>SGSVTAGMALAATDIPGLDASKLVSGVLAEQRLPVFARGLATAVSNSSDPNTATVPLMLTNHANGPVAGRYFYIQSMFYPDQNGNASQIATSYNATSEMYVRVSYAANPSIREWLPWQRCDIGGSFTKEADGELPGGVNLDSMVTSGWWSQSFTAQAASGANYPIVRAGLLHVYAASSNFIYQTYQAYDGESFYFRCRHSNTWFPWRRMWHGGDFNPSDYLLKSGFYWNALPGKPATFPPSAHNHDVGQLTSGILPLARGGVGSNTAAGARSTIGAGVPATASLGASGWWRDNDTGLIRQWGQVTCPADADASITFPIPFPTLCLGGYANQTSAFHPGTDASTGF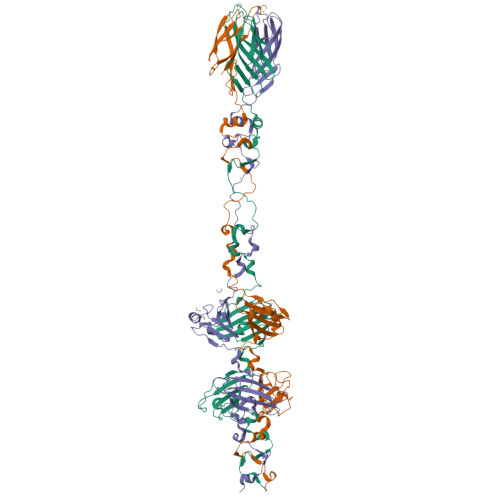RGATTTTAVIRNGYFAQAVLSWEAFGR[6x]> 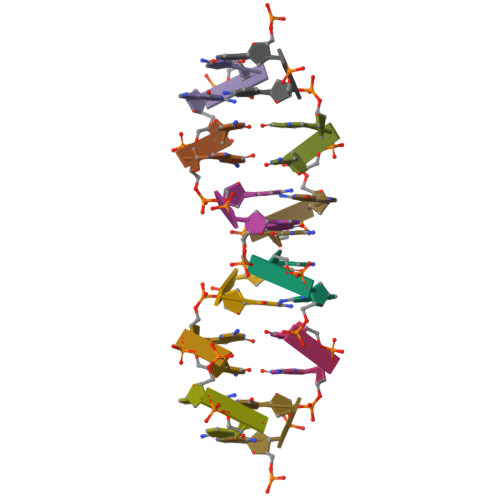GC> TGMSREEVESLIQEVLEVYPEKARKDRNK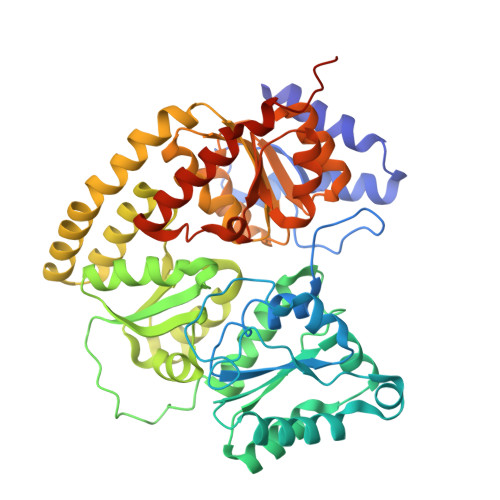HLAVNDPAVTQSKKCIISNKKSQPGLMTIRGCAYAGSKGVVWGPIKDMIHISHGPVGCGQYSRAGRRNYYIGTTGVNAFVTMNFTSDFQEKDIVFGGDKKLAKLIDEVETLFPLNKGISVQSECPIGLIGDDIESVSKVKGAELSKTIVPVRCEGFRGVSQSLGHHIANDAVRDWVLGKRDEDTTFASTPYDVAIIGDYNIGGDAWSSRILLEEMGLRCVAQWSGDGSISEIELTPKVKLNLVHCYRSMNYISRHMEEKYGIPWMEYNFFGPTKTIESLRAIAAKFDESIQKKCEEVIAKYKPEWEAVVAKYRPRLEGKRVMLYIGGLRPRHVIGAYEDLGMEVVGTGYEFAHNDDYDRTMKEMGDSTLLYDDVTGYEFEEFVKRIKPDLIGSGIKEKFIFQKMGIPFREMHSWDYSGPYHGFDGFAIFARDMDMTLNNPCWKKLQAPWEASEGAEKVAASA The β-lactamase of Mycobacterium tuberculosis, BlaC, is susceptible to inhibition by clavulanic acid. One of the most conserved motifs in class A β-lactamase active sites is the serine-aspartate-asparagine (SDN) motif at Ambler positions 130 to 132. In BlaC, however, the asparagine at position 132 is replaced by a glycine. This substitution effectively removes a side chain with an amide functional group from the active-site pocket, resulting in an enlarged active site in BlaC.

BlaC G132N gave crystals useful for X-ray diffraction, resulting in a structure at a 1.6-Å resolution and Rwork/Rfree factor values of 15.5/18.8%. The structure is overall similar to that of wt BlaC, but notable differences exist. The Asn side chain that is introduced at position 132 occupies the canonical position for class A β-lactamases (e.g., in TEM-1 and SHV-1). The oxygen of the side chain is hydrogen bonded (2.7 Å) with the amide of Lys73. Strikingly, however, the nitrogen of the Asn132 side chain hydrogen bonds (2.8 Å) to the carbonyl oxygen of residue Ser104. This bond flips the carbonyl of Ser104 and forces it into a cis-peptide conformation. An interesting double conformation is also observed for the Ser130 side chain. This side chain in the BlaC G132N structure has roughly 50% occupation of the canonical position that is observed in all but six homologues in the PDB, donating a hydrogen toward a bond to the conserved active-site phosphate (2.6 Å) and perhaps receiving a hydrogen from the Lys234 amide (2.9 Å). The multiple conformations for BlaC G132N could at least partially be propagated through Ser104-Ile105 peptide bond isomerization and are suggestive of increased dynamics relative to the wild-type enzyme.

> GADLADRFAELERRYDARLGVYVPATGTTAAIEYRADERFAFCSTFKAPLVAAVLHQNPLTHLDKLITYTSDDIRSISPVAQQHVQTGMTIGQLCDAAIRYSDNTAANLLLADLGGPGGGTAAFTGYLRSLGDTVSRLDAEEPELNRDPPGDERDTTTPHAIALVLQQLVLGNALPPDKRALLTDWMARNTTGAKRIRAGFPADWKVIDKTGTGDYGRANDIAVVWSPTGVPYVVAVMSDRAGGGYDAEPREALLAEAATCVAGVLA>[2x]METIQELILSEENKTNIAVLNLGTNDRRNAVLILETALHLVEKYLGKIINTSYLYETVPEYIVLDKKESCEKINKDCRIYDVNYINELMQNLEESKYEENKELIDKCEEYETFLKNGKVDNSILKEVNVENYLLECNNIIVKNDEIMKNNLSKYKDKYYTSYFYNLTVVVKTFVNDPLSMLVVIKYIEELMKRENVKEKEKFENRIIDIDILFFNDFTIFMKNIKLEKNMIYKILSKYIHLERDIKNGNDNMSKVNMDKDINLNNNNNIKKKNNNDIDCDCVDQKMNNHVNNKNYINSFRDPQEIINNMVDNIEFLSIPHVYTTHRYSILLCLNDMIPEYKHNVLNN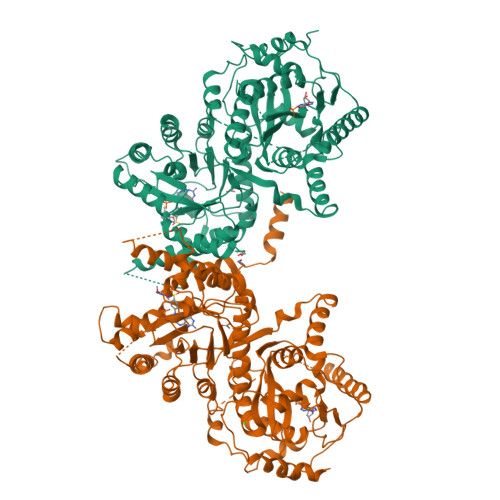TIRCLYNKYVSRMKEQYNINIKENNKRIYVLKDRISYLKEKTNIVGILNVNYDSFSDGGIFVEPKRAVQRMFEMINEGASVIDIGGESFGPFVIPNPKISERDLVVPVLQLFQKEWNDIKNKIVKCDAKPIISIDTINYNVFKECVDNDLVDILNDISACTNNPEIIKLLKKKNKFYSVVLMHKRGNPHTMDKLTNYDNLVYDIKNYLEQRLNFLVLNGIPRYRILFDIGLGFAKKHDQSIKLLQNIHVYDEYPLFIGYSRKRFISHCMNDQNVVINTQQKLHDEQQNENKNIVDKSHNWMFQMNYMRKDKDQLLYQKNICGGLAIASYSYYKKVDLIRVHDVLETKSVLDVLTKIDQVKDPNSSSVDKLAAALEHHHHHH> SHIEGYECQPIFLNVLEAIEPGVVCAGHDNNQPDSFAALLSSLNELGERQLVHVVKWAKALPGFRNLHVDDQMAVIQYSW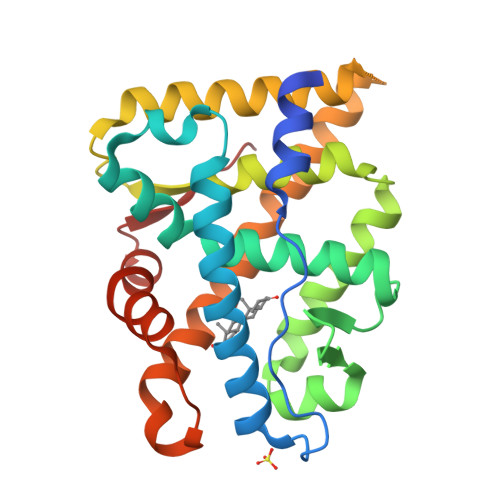MGLMVFAMGWRSFTNVNSRMLYFAPDLVFNEYRMHKSRMYSQCVRMRHLSQEFGWLQITPQEFLCMKALLLFSIIPVDGLKNQKFFDELRMNYIKELDRIIACKRKNPTSCSRRFYQLTKLLDSVQPIARELYQLAFDLLIKSHMVSVDFPEMMAEIISVQVPKILSGKVKPIYFHTQ The use of cyanuric acid hydrolase to solve this societal problem is being explored and the best candidate for this biotechnological application is the thermostable enzyme from Moorella thermoacetica. Consistent with the “Toblerone fold” observed for these enzymes[8–10], the RMCAH monomer is composed of three concatenated, highly divergent, but structurally homologous domains, which endows the enzyme monomer an internal pseudo-three-fold symmetry (Domains 1, 2). As observed for AtzD and ACAH, the active site of RMCAH lies on the pseudo-three-fold axis within each monomer and is formed by similar sets of residues from all three domains. As observed for ACAH and AtzD, each of the three serine γO atoms is in close proximity to a lysine residue (Lys40, Lys161 and Lys299), generating three pairs of Ser-Lys dyads each from one of the three isostructural domains from the same monomer.

To further probe functional importance of the domain 2 flexibility, we generated a double-mutant enzyme ‘RMCAH-CC’ (G53C/E235C) in which Gly53 and Glu253 from domain 1 and 2, respectively, have been changed to Cys. We confirmed that these two cysteines introduced near the domain1/2 interface can form a disulfide bond, by determining a crystal structure of RMCAH with several additional mutations C46S/C162A/C218V/G53C/E235C. This structure showed the domain 2 locked in a partially open conformation via the disulfide linkage. Notably, RMCAH-CC showed higher activity in the presence of 10 mM DTT than in the absence of DTT. This was in contrast to wild-type RMCAH that was slightly inhibited by the high concentration of DTT possibly due to an adduct formation involving cysteine residues near the active site.

>MQKVEVFRIPTASPDDISGLATLIDSGKINPAEIVAILGKTEGNGSVNDFTRCFATQSLAMYLAEKLGISREEVVKKVAFIMSGGTEGVMTPHITVFVRKDVAAPAAPGKRLAVGVAFTRDFLPEELGRMEQVNEVARAVKEAMKDAQIDDPRDVHFVQIKAPLLTAERIEDAKRRGKDVVVNDTYKSMAYSRGASALGVALALGEISADKISNEAIVHDWNLYSSVASTSAGVCLLNDEIIVVGNSTNSASDLVIGHSVMKDAIDADAVRAALKDAGIRSDDEMDRIVNVLAKAEAASSGTVRGRRNTMLDDSDINHTRSARAVVNAVIASVVGDPMVYVSGGAEHQGPDGGGPIAVIARVLEHHHHHH[8x]>[4x]MTSFTIPGLSDKKASDVADLLQKQLSTYNDLHLTLKHVHWNVVGPNFIGVHEMIDPQVELVRGYADEVAERIATL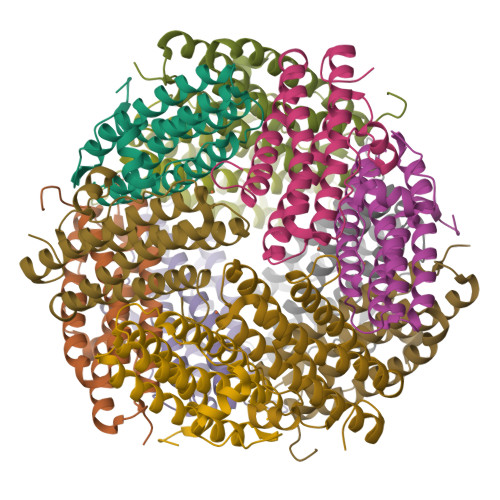GKSPKGTPGAIIKDRTWDDYSVERDTVQAHLAALDLVYNGVIEDTRKSIEKLEDLDLVSQDLLIAHAGELEKFQWFVRAHLESAGGQLTHEGQSTEKGAADKARRKSA>MRMSDGAAPKANGSEASGQDLVPAAVEQAVPIQPVAGAALAAPAAGQINQIDPWIFQNFVQCPLGEFSISPRNTPGEILFDLALGPGLNPYLAHLSAMYTGWV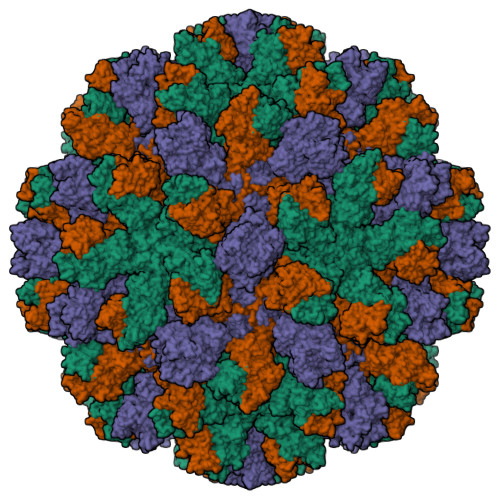GNMEVQLVLAGNAFTAGKVVVALVPPYFPKGSLTTAQITCFPHVMCDVRTLEPIQLPLLDVRRVLWHATQDQEESMRLVCMLYTPLRTNSPGDESFVVSGRLLSKPAADFNFVYLTPPIERTIYRMVDLPVIQPRLCTHARWPAPVYGLLVDPSLPSNPQWQNGRVHVDGTLLGTTPISGSWVSCFAAEAAYKFQSGTGEVATFTLIEQDGSAYVPGDRAAPLGYPDFSGQLEIEVQTETTKTGDKLKVTTFEMILGPTTNADQAPYQGRVFASVTAAASLDLVDGRVRAVPRSIYGFQDTIPEYNDGLLVPLAPPIGPFLPGEVLLRFRTYMRQIDTADAAAEAIDCALPQEFVSWFASNAFTVQSEALLLRYRNTLTGQLLFECKLYNEGYIALSYSGSGPLTFPTDGIFEVVSWVPRLYQLASVGSLATGRMLKQ[3x]> MGIRELNLTKEQHEWLNGWLELWGAWVYSGRLEKRMSSVIAKFMESVEPGRVMTRPMCNDDDGMLI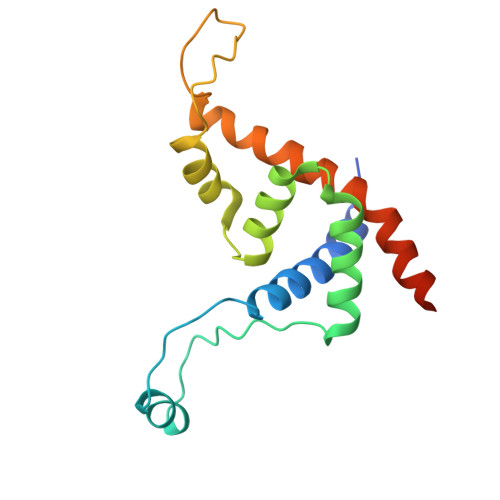SQVVDSVMYIDKKAFGILLSYYAHGSSKHAIASYYHRVARPRKMLCRGGGRIQKPSLATCRREVDEILNASLFMIYPVLDSAFKNRKRVEKIKHVA In Drosophila, an RNase III enzyme Dicer-2 (Dcr-2), aided by its cofactor Loquacious-PD (Loqs-PD), has an important role in generating 21 bp siRNA duplexes from long double-stranded RNAs (dsRNAs). ATP hydrolysis by the helicase domain of Dcr-2 is critical to the successful processing of a long dsRNA into consecutive siRNA duplexes. Here six cryo-electron microscopy (cryo-EM) structures of Drosophila Dcr-2–Loqs-PD in apo and in complex with dsRNA substrate in the absence or in the presence of ATP were captured, illuminating the continuous conformational changes of Dcr-2–Loqs-PD after binding to dsRNA and translocating until forming the active dicing state and cleaving the dsRNA substrate into an siRNA duplex in the post-dicing state. Loqs-PD is a cofactor protein that comprises two dsRBDs that are responsible for recruiting siRNA precursor substrates for Dcr-2.

Similar to human Dicer, the N-terminal helicase region forms the base of the L-shaped structure and the DUF283 domain is located at the corner of the L and just below the catalytic active core. The previously unmodelled linker between the DUF283 and Platform domains (DP-linker) in human Dicer is now well resolved in Dcr-2 as a structural element that interacts with the RNase IIIa domain through two α-helices and one β-strand. The Platform and PAZ domains surrounding the Connector helix sit at the top of the core processing region. The intrinsic RNase III dimer comprising the RIIIDa and RIIIDb domains is located in the centre of the molecule with the insertion domains (RIIIDai and RIIIDbi) sitting in symmetric positions. The C-terminal dsRBD interacts with the DP-linker and shields the RNase-activity centre. Compared with the apo state, the overall structures of Dcr-2–Loqs-PD complex undergo major conformational changes when interacting with the dsRNA substrate, especially on the helicase and DUF283 domains. Although we cannot conclude whether the dimerization is an in vitro artifact or whether it is physiologically relevant, this finding helped us to solve near-atomic high-resolution structures of Dcr-2–Loqs-PD in the apo and initial binding states under conditions without ATP.

> MEDVEIKPRGYQLRLVDHLTKSNGIVYLPTGSGKTFVAILVLKRFSQDFDKPIESGGKRALFMCNTVELARQQAMAVRRCTNFKVGFYVGEQGVDDWTRGMWSDEIKKNQVLVGTAQVFLDMVTQTYVALSSLSVVIIDECHHGTGHHPFREFMRLFTIANQTKLPRVVGLTGVLIKGNEITNVATKLKELEITYRGNIITVSDTKEMENVMLYATKPTEVMVSFPHQEQVLTVTRLISAEIEKFYVSLDLMNIGVQPIRRSKSLQCLRDPSKKSFVKQLFNDFLYQMKEYGIYAASIAIISLIVEFDIKRRQAETLSVKLMHRTALTLCEKIRHLLVQKLQDMTYDDDDDNVNTEEVIMNFSTPKVQRFLMSLKVSFADKDPKDICCLVFVERRYTCKCIYGLLLNYIQSTPELRNVLTPQFMVGRNNISPDFESVLERKWQKSAIQQFRDGNANLMICSSVLEEGIDVQACNHVFILDPVKTFNMYVQSKGRARTTEAKFVLFTADKEREKTIQQIYQYRKAHNDIAEYLKDRVLEKTEPELYEIKGHFQDDIDPFTNENGAVLLPNNALAILHRYCQTIPTDAFGFVIPWFHVLQEDERDRIFGVSAKGKHVISINMPVNCMLRDTIYSDPMDNVKTAKISAAFKACKVLYSLGELNERFVPKTLKERVASIADVHFEHWNKYGDSVTATVNKADKSKDRTYKTECPLEFYDALPRVGEICYAYEIFLEPQFESCEYTEHMYLNLQTPRNYAILLRNKLPRLAEMPLFSNQGKLHVRVANAPLEVIIQNSEQLELLHQFHGMVFRDILKIWHPFFVLDRRSKENSYLVVPLILGAGEQKCFDWELMTNFRRLPQSHGSNVQQREQQPAPRPEDFEGKIVTQWYANYDKPMLVTKVHRELTPLSYMEKNQQDKTYYEFTMSKYGNRIGDVVHKDKFMIEVRDLTEQLTFYVHNRGKFNAKSKAKMKVILIPELCFNFNFPGDLWLKLIFLPSILNRMYFLLHAEALRKRFNTYLNLHLLPFNGTDYMPRPLEIDYSLKRNVDPLGNVIPTEDIEEPKSLLEPMPTKSIEASVANLEITEFENPWQKYMEPVDLSRNLLSTYPVELDYYYHFSVGNVCEMNEMDFEDKEYWAKNQFHMPTGNIYGNRTPAKTNANVPALMPSKPTVRGKVKPLLILQKTVSKEHITPAEQGEFLAAITASSAADVFDMERLEILGNSFLKLSATLYLASKYSDWNEGTLTEVKSKLVSNRNLLFCLIDADIPKTLNTIQFTPRYTWLPPGISLPHNVLALWRENPEFAKIIGPHNLRDLALGDEESLVKGNCSDINYNRFVEGCRANGQSFYAGADFSSEVNFCVGLVTIPNKVIADTLEALLGVIVKNYGLQHAFKMLEYFKICRADIDKPLTQLLNLELGGKKMRANVNTTEIDGFLINHYYLEKNLGYTFKDRRYLLQALTHPSYPTNRITGSYQELEFIGNAILDFLISAYIFENNTKMNPGALTDLRSALVNNTTLACICVRHRLHFFILAENAKLSEIISKFVNFQESQGHRVTNYVRILLEEADVQPTPLDLDDELDMTELPHANKCISQEAEKGVPPKGEFNMSTNVDVPKALGDVLEALIAAVYLDCRDLQRTWEVIFNLFEPELQEFTRKVPINHIRQLVEHKHAKPVFSSPIVEGETVMVSCQFTCMEKTIKVYGFGSNKDQAKLSAAKHALQQLSKCDA;> MDQENFHGSSLPQQLQNLHIQPQQASPNPVQTGFAPRRHYNNLVGLGNGNAVSGSPVKGAPLGQRHVKLKKEKISAQVAQLSQPGQLQLSDVGDPALAGGSGLQGGVGLMGVILPSDEALKFVSETDANGLAMKTPVSILQELLSRRGITPGYELVQIEGAIHEPTFRFRVSFKDKDTPFTAMGAGRSKKEAKHAAARALIDKLIGAQLPESPSSSAGPSVTGLTVAGSGGDGNANATGGGDASDKTVGNPIGWLQEMCMQRRWPPPSYETETEVGLPHERLFTIACSILNYREMGKGKSKKIAKRLAAHRMWMRLQETPIDSGKISDSICGELEGEVSIIQDIDRYEQVSKDFEFIKI> GCAGCC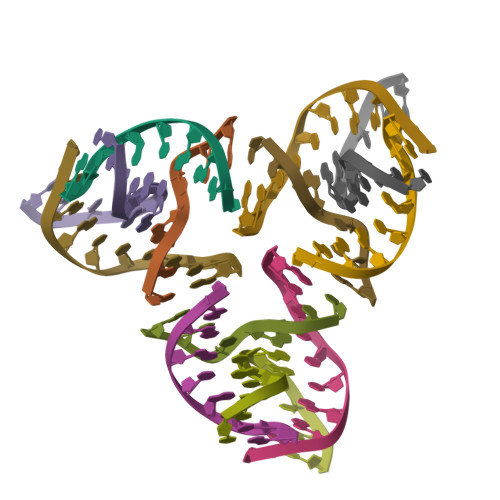TGTA;> TACACCG;> TGATGTGGCTGC;> CGGACATCA> MQCHHNVLVGWANSGSSTAAFLTQQQQQPLPPSPLRFLWADQPLGSPSVLAPGCGMYRARSCGVVAASAAAPRVRTALDMVIRSYTPIYAPDPATDHLGALRSADECRTLWAQHIPVPSLTRAIELWLRFGNDPVVHTAASTASAERAEGDAAPSSTSPFAYVEDYMGSNMVTGTPEHVKESAELWSEYFETKYVRRMRQSRRTSKQYVGVLGAAGRGRGAGESGGGSASSSIANLLLDEADHPNTKWEADTFFCEVAYLSERHLKTRVTNHLQLDKLLW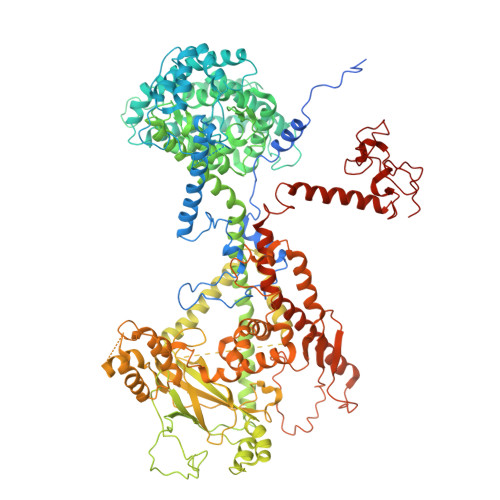GGTAKPDAFVQFFEAFQQQTITRIPLPVPSIWVHESTEAKKKWAEHYLPACSAAHEFFQEKLRPHAADAAAQAKLLADVAAAYRQVHAILLERRARQVQAGVYPSTWTGGGAAATATEEAWAANEAEKEQRRMDEGVYDPEDLLDTTAEWATEHAKIQAILEQPLTSSGSNGEKSYGFSLQDFWLHTERREALETVHVLESESLARVAAAARRRLYSETPLPDVFAGLEESVAKARLDLRAAVLKPHFNSVWCRMHYVKFGAASLVQHTHTASRQLLFHYAASTQVVAATAEMYYATKPLSSQLDYASPYTFRRSLARHCTRYGVEMAHAAQQPLLLSAAYLAKAEGVIGRVARQAAAPFGARRRARYSAAQLNNQRLLNPVKSVQVTAPAPELLAAGADLLTILREERTPKAKAAGEALKVWPLGSRQTVSYDWTSPALDKLRLTDSSLTAEQAAQRDQLRQAGRLEISLWRRRTAEERQKVRAEMKKEAVDVQALVAETPVLQEVLAYASHLYRKLTREQEQEQSYSDTVPTPHAWDEASGEWVFAVMLDDDVPLSETQSTEVFLPYVDAAGRRLPNGEYRVAVRAVDRELNPTEHPTLMSAATSSPFSVVDALPQLYAQYTRHPQPADKATGTPTEAPLEGDVAGKDLMSFCAFLREAGLHISLSAEFAMGQSLDKQGNVSVAEVAAVLRGTEYHRSQCEHGITDAQRTIEPQCRLHWSLYHPGATEQEWAAARRRVLRRAMAEERDWWLPDPMLEVTDVRTDSAGAASFSFGAYPAVARYGTELCTVLPAHGSNHMEYAVLPPPPGVKATARGIGAQVQAECTVDGTGAIASLHYGAPISAADVTVEDALRAAMEAIQVAQMRHNTLSMVKLCAFEKQAQTMLFCGIQGLEFGGKHGRTYAYALEKAKREMAATAEAGQVASLQAADAEKLRLSDQEQTSAAVDRFASQTNPEQRLTRFVPRSTMSGYSMEDVGPERASTWGL> SMQQDIVNDHQEEAQGWKWEQIKEIIESGELARLKRSRQMTDKYHEHKKRTAGLDMNQYVLQKLGWS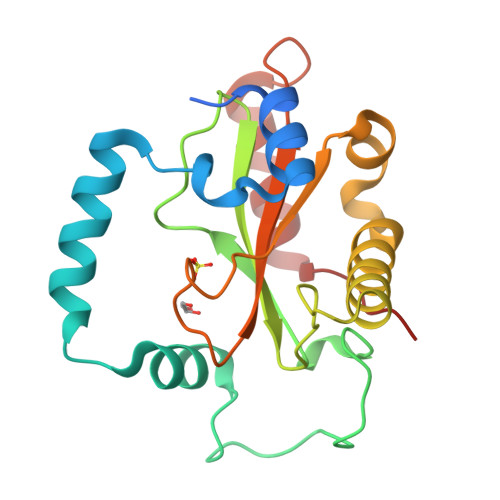LDEPQLENAAAKAFSSSTLYAVRANDFPYNFEPGVVHLVLWSKVALPVHSPDKAVREAARARMNAFLQAQPLLRPLLSSGHVAWFVNYPELQSVARIFHAHVLLFFPRERYSAEQVKTTVDDILSHGFEPLA> MSSGNSSLGIIVGIDDSPAAQVAVRWAARDAELRKIPLTLVHAVSPEVATWLEVPLPPGVLRWQQDHGRHLIDDALKVVEQASLRAGPPTVHSEIVPAAAVPTLVDMSKDAVLMVVGCLGSGRWPGRLLGSVSSGLLRHAHCPVVIIHDEDSVMPHPQQAPVLVGVDGSSASELATAIAFDEA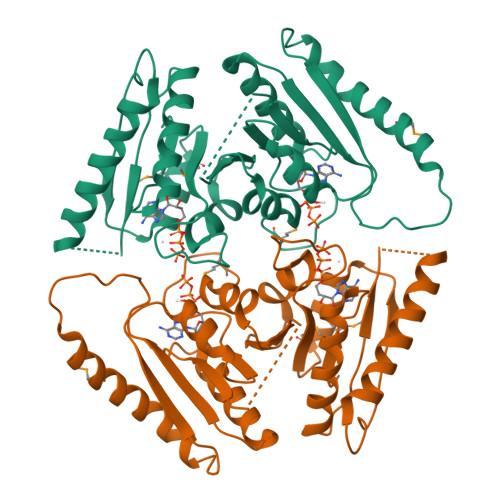SRRNVDLVALHAWSDVDVSEWPGIDWPATQSMAEQVLAERLAGWQERYPNVAITRVVVRDQPARQLVQRSEEAQLVVVGSRGRGGYAGMLVGSVGETVAQLARTPVIVARESLTLEHHHHHH>[2x]MKILITGGAGFIGSAVVRHIIKNTQDTVVNIDKLTYAGNLESLSDISESNRYNFEHADICDSAEITRIFEQYQPDAVMHLAAESHVDRSITGPAAFIETNIVGTYALLEVARKYWSALGEDKKNNFRFHHISTDEVYGDLPHPDEVENSVTLPLFTETTAYAPSSPYSASKASSDHLVRAWRRTYGLPTIVTNCSNNYGPYHFPEKLIPLVILNALEGKPLPIYGK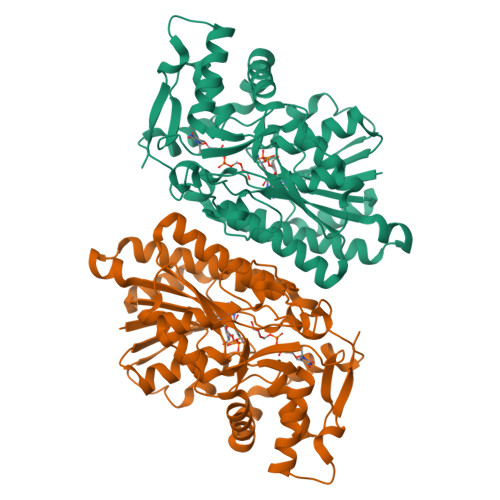GDQIRDWLYVEDHARALHMVVTEGKAGETYNIGGHNEKKNLDVVFTICDLLDEIVPKATSYREQITYVADRPGHDRRYAIDAGKISRELGWKPLETFESGIRKTVEWYLANTQWVNNVKSGAYQSWIEQNYEGRQ>MHHHHHHGGNMISYALLGVILGISGVIYAVYLAVWVLRQDPGNEKMRFISQAIATGARAYLFRQYRTLAVLLVILAVLILVAIDMPRRTFGLTALAFIVGALGSMLAGYLGMYVTTRSASRVAQAAATGGMGKALLVSWRAGAVMGLSLASIALLLISGFYLVFRSVLPDDWAVPLVALGFGASLVTLFMRVGGGIYTKAADLGADLVGKVEAGIPEDDPRNPGVIADNVGDNVGDVAGMAADVYESYIVTVTAAIFLAAILGLPTQFIEAIILFAALALVATFAGVNLLKTTGVKHPLSSISLAIYATIGLSVVLFFIGAFTLGLDSTKALALAATTSLGAVIAPLIVKITDYYTSYNYGPVRKIAEQAKISPATVIITGYGVGLMSAIPVIAVIVAVLGISYMIGYYTVPVSGFGELSKYLAGIFGTAMASVGLLVVAGIIITADSYGPVSDNAGGVVEMAGLPDEVREITDVLDSVGNTTKATTKGYAIASAALAALVLFIALIFEIVYSASKILGKGIVDMISESLSGLQLINANVLIGAFLGVALVYFFSSRTLEAVGRTAMEIVEEIRRQFREKPGILEWKEQPDYARVVDIATRRALGEFLIPGLAAIVLPLITGLLLGWNALAGLIMGAIVAGVPRALLMANAGGAWDNAKKYIEIQGLKKTEMHKAAVIGDTVGDPMKDTVGPSLNPLIKVLNTLSVVFTYVIVSTNIALGIWPSGLLPF[2x]

Membrane-bound pyrophosphatases (M-PPases) are homodimeric primary ion pumps that couple the transport of Na+- and/or H+ across membranes to the hydrolysis of pyrophosphate. M-PPases are large (66–89 kDa), single-domain integral membrane proteins comprised of two identical monomers, each with 15–17 transmembrane helices. The helices of each subunit arrange into an inner ring (helices 5, 6, 11, 12, 15, 16) containing the functional core (active site, coupling funnel, ion gate, exit channel) and an outer ring (helices 1–4, 7–10, 13, 14) of largely unknown function. To date, H+-pumping (H+-PPase), Na+-pumping (Na+-PPase) and dual-pumping (Na+,H+-PPase) M-PPases have been found, most of which require potassium (K+) for maximal catalytic activity.

To address them, we solved the first structure of a K+-independent M-PPase (from the thermophile Pyrobaculum aerophilum, PaPPase), performed enzymatic assays on native PaPPase and three variants (A12.46K and A12.49T, and the double mutant), and conducted both electrometric and time-resolved crystallographic studies on TmPPase, a K+-dependent Na+-PPase. The PaPPase structure is in the Mg5IDP-bound state with loop closed and a structural water located at the ion gate. In our new structure, the E5.71-R13.62-R/I/Kˈ10.33 interaction is lost: the cytoplasmic regions of helices 13–14 are straightened (Fig. EV1B), resembling resting state (Fig. EV1C) and product-bound (Fig. EV1D,E) structures despite having IDP bound. Helix 5 is straighter than in other M-PPases, which also straightens helices 13–14 (cytoplasmic side) and 2–3 (periplasmic side) by pushing them away from the inner ring. Our PaPPase:Mg5IDP structure provides the first data on the ion gate set-up of K+-independent H+-PPases with E6.53 and shows that the 3D orientation of ion gate residues D6.50, S6.54, N16.46 and E6.53 in particular all resemble the structure of VrPPase:Mg5IDP, a H+-pump with E6.57, and not TmPPase:Mg5IDP, a Na+-pump with E6.53, despite the shift of the semi-conserved glutamate. We modelled SO42− from the crystallisation solution to mediate the inter-subunit communication of Y10.44, Y13.44, and R15.40 in PaPPase:Mg5IDP, but this may be Pi (not present in crystallisation) under physiological conditions. For K12.46, this indeed places ε-NH3+ of K12.46 at the K+-binding site, which would explain K+-independence.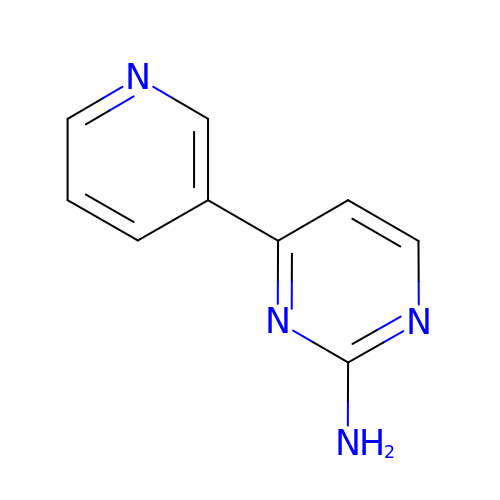2-AMINO-4-PYRIDYL-PYRIMIDINE | C9 H8 N4 | LQHQKYWYKPLKCH-UHFFFAOYSA-N> AAPTAYTPLDVAQAY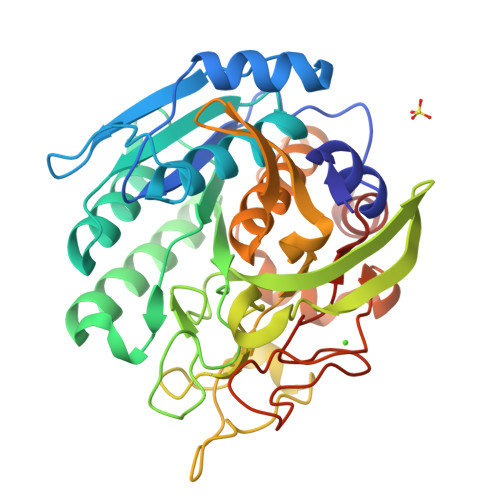QFPEGLDGQGQCIAIIELGGGYDEASLAQYFASLGVPAPQVVSVSVDGASNQPTGDPSGPDGEVELDIEVAGALAPGAKFAVYFAPNTDAGFLDAITTAIHDPTLKPSVVSISWGGPEDSWTSAAIAAMNRAFLDAAALGVTVLAAAGNSGSTDGEQDGLYHVDFPAASPYVLACGGTRLVASGGRIAQETVWNDGPDGGATGGGVSRIFPLPAWQEHANVPPSANPGASSGRGVPDLAGNADPATGYEVVIDGEATVIGGTSAVAPLFAALVARINQKLGKAVGYLNPTLYQLPADVFHDITEGNNDIANRAQIYQAGPGWDPCTGLGSPIGVRLLQALLPSASQPQP> MTNIIQADEPTTLTTNALDLNSVLGKDYGALKDIVINANPASPPLSLLVLHRLLCEHFRVLSTVHTHDSVK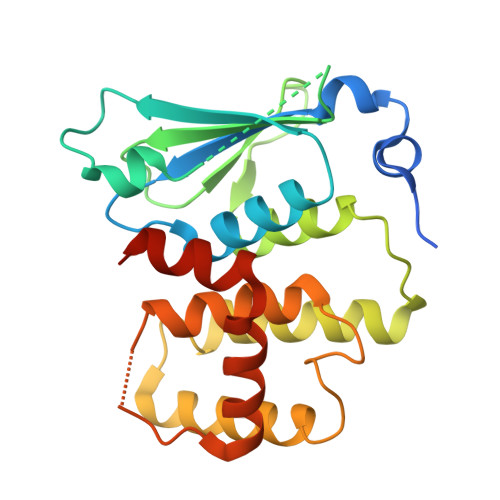SVPENLLKCFGEQNKKQPRQDYQLGFTLIWKNVPKTQMKFSIQTMCPIEGEGNIARFLFSLFGQKHNAVNATLIDSWVDIAIFQLKEGSSKEKAAVFRSMNSALGKSPWLAGNELTVADVVLWSVLQQIGGCSVTVPANVQRWMRSCENLAPFNTALKLLKLEHHHHHH>GPLGSMFDIKRKTIEWGGKTLVLETGRIARQADGAVLATMGETVVLATAVFAKSQKPGQDFFPLTVNYQEKTFAAGKIPGGFFKREGRPSEKETLVSRLIDRPIRPLFVKGFKNEVQVVVTVLQHDLENDPDILGMVAASAALCLSGAPFMGPIGAARVGWVDGAYVLNPTLDEMKESKMDLVVAGTADAVMMVESEIQELSEEIVLGGVNFAHQQMQAVIDAIIDLAEHAAKEPFAFEPEDTDAIKAKMKDLVGADIAAAYKIQKKQDRYEAVGAAKKKAIAALGLSDENPTGYDPLKLGAIFKELEADVVRRGILDTGLRIDGRDVKTVRPILGEVGILPRTHGSALFTRGETQAIVVATLGTGDDEQFIDALEGTYKESFLLHYNFPPYSVGETGRMGSPGRREIGHGKLAWRALRPMLPTKEDFPYTIRLVSEITESNGSSSMATVCGSSLAMMDAGVPLVRPVSGIAMGLILEQDGFAVLSDILGDEDHLGDMDFKVAGTSEGLTSLQMDIKIAGITPAIMEQALAQAKEGRAHILGEMNKAMDAPRADVGDFAPKIETINIPTDKIREVIGSGGKVIREIVATTGAKVDINDDGVVKVSASDGAKIKAAIDWIKSITDEAEVGKIYDGKVVKVVDFGAFVNFFGAKDGLVHVSQISNERVAKPSDVLKEGQMVKVKLLGFDDRGKTKLSMKVVDQETGEDLSKKEAAAEEA[3x]

The phosphorolytic exoribonuclease polynucleotide phosphorylase (PNPase; EC 2.7.7.8) is encoded in the genomes of bacteria and eukaryotes, and in those domains of life the ribonuclease plays multifaceted roles in regulation and environmental response. While the C-terminal RNase PH-like domain catalyses phosphorolytic attack of RNA, the N-terminal domain has lost this capacity; instead, it contributes to the ring-like quaternary structure of the trimeric PNPase assembly. Two recurrent structural motifs that are found in many RNA-binding proteins, the S1 and K-homology (KH) domains, are appended at the C-terminus of PNPase. The PNPase studied here is from the bacterium Caulobacter crescentus, which has been established as a model system to investigate cell cycle progression, because populations can be readily prepared that are synchronized in the cell cycle.

Crystals of the RNA-bound material were obtained in space group P22121 that contain a PNPase trimer in the asymmetric unit. The other two KH domains were found in the unbiased maps. It was also clear from the early electron density maps that RNA was present and interacting with the KH domains. The refined crystal structure revealed 12 RNA nucleotides, and while it was anticipated that 20–30 oligonucleotides would be present in the structure based on spectroscopic absorbance, the RNA may have been partially degraded during crystallization or may be extensively disordered in some places. The S1 domains are therefore apparently disordered in the RNA-bound structure. The three KH domains (residues 556–619) interact with the RNA in the manner of three overlapping hands grasping a length of rope. The RNA follows a spiralling trajectory, with bases on the outside and phosphate backbone innermost. The path of the RNA continues from the KH ensemble to the aperture of the central channel, where a base stacks on the aromatic side chain of the conserved FF loop. The KH domains adopt non-equivalent orientations with respect to the RNase PH-like core, and each domain contacts the RNA at different points. However, the structure suggests that the 3′–5′ polarity of the substrate originates from the interactions of the GSGG loops with the RNA sugar–phosphate backbone by the KH domains.>QLLGLLGQAATVIGGEPTVSVEQLDFSAARGDVALQVRAPGFDVLERLRSRLSESGLAVQLGSASRDGSTV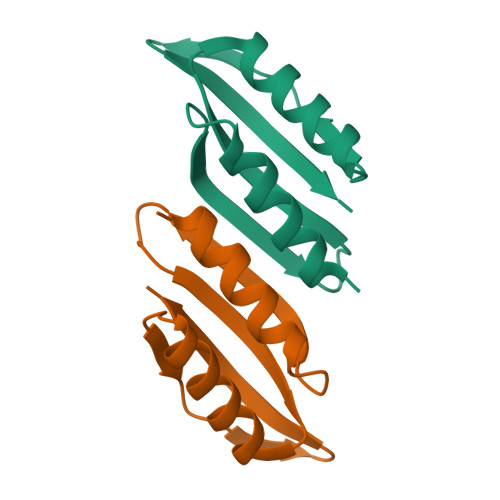SARLVIG[2x]> GWMWNQFFLLEEYTGSDYQYVGKLHSDQDKGDGSLKYILSGDGAGTLFIIDEKTGDIHATRRIDREEKAFYTLRAQAIN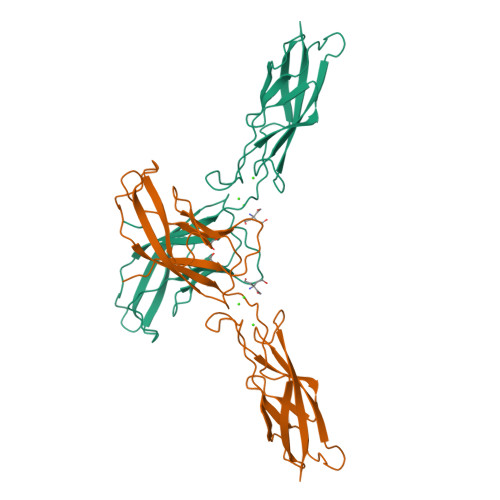RRTLRPVEPESEFVIKIHDINDNEPTFPEEIYTASVPEMSVVGTSVVQVTATDADDPSYGNSARVIYSILQGQPYFSVEPETGIIRTALPNMNRENKEQYQVVIQAKDMGGQMGGLSGTTTVNITLTD Here, we report a δ-poly-L-ornithine synthetase from Acinetobacter baumannii, which we name PosA. Nonribosomal peptide synthetase (NRPS) enzymes, usually composed of condensation, adenylation, and thiolation domains, are involved in peptide natural product biosynthesis to produce antibiotics and siderophores. Activity analyses show that the A. baumannii homolog activates L-Orn and the full-length protein produces isopeptide polymers in vitro. Structures of the isolated adenylation domain from PosA are presented with several diamino acids and biochemical assays identify important substrate binding residues.

To better understand the substrate binding in PosA, we solved four structures of the isolated adenylation domain. Substrates bind at the center of the core adenylation domain where residues mainly from subdomain I mediate binding. Glu221 showed charged interaction with terminal δ-amine of ornithine substrates or the ε-amino group of lysine indicating an important role in binding. The polar side chains of Thr304 and Ser313 were also found to be placed at hydrogen bonding distances of 2.9 and 2.6 Å from the terminal amine group of L-ornithine. The structures with substrates revealed Asp217, Met218, Glu221, Thr304, and Ser313 as interacting residues with the diamine substrates. Mutation of individual residues showed Asp217 and Glu221 were the most important residues for substrate activation since no enzymatic activity was observed in these mutants even at high protein or substrate concentration. Removal of the hydroxyl group from the side chains of Thr304 and Ser313 showed 33- and 183-fold reduction in catalytic efficiency in T304A and S313A mutants, respectively, indicating these residues are also important for binding. The enzyme assay with L-ornithine showed the highest activity while low activity was observed with DAB. This suggested L-ornithine was the most preferred substrate for the εPLs homolog from A. baumannii.

>[2x]GHMNQFVTNTKNVIRGKYHPEFLQNEVLADIFAHTAQTLPDKTALIEADKTLSYGELYQQALIMAQHLALKGVKPGHIVGLWLPRGIELLKAQLAICLSGAAWLPFDMDTPADRIAVCLEDAEAVGMITTDEWYEHLAEVPQTKWTNTELQKPLSESVSLAKTTPDQPAYIIYTSGSTGKPKGIVITQKNICHFLRSENSILGIQEQDKVYQGFSVAFDMSFEEIWLSYLVGATLWIAPKSLVSDPERLCQTLKQEQITVLHAVPTLLALFPEDVPNLRIINLGGEMCPDSLVDRWALPHHQMFNTYGPTETTVSASLELLERGKPVTIGKPLPNYGMLVINSERELLEQGETGELCIFGPSVAQGYLGRPDLTADKFIENPWAMSVEEELLYRTGDLAKIDEFGQVHCLGRAD>GPLGSQEQKQMLGERLFPLIQAMHPTLAGKITGMLLEIDNSELLHMLESPESLRSKVDEAVAVLQAHQAKEAAQKA[8x];>[8x]SNLNPNAPEFHPGVPWKG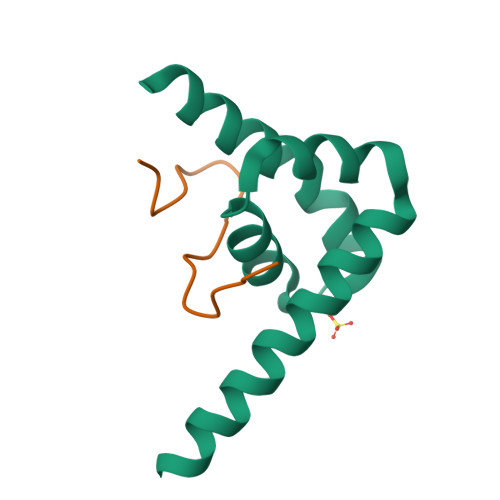LQNI>[2x]MSKNKVVIIGAGFAGLVAARELQTAGIEYEILEAKDRIGGRAWTEERMGRPLELGATWVHWFQAHTWTEIMRYGQRTEITASPSGNDAHWVTDGKVV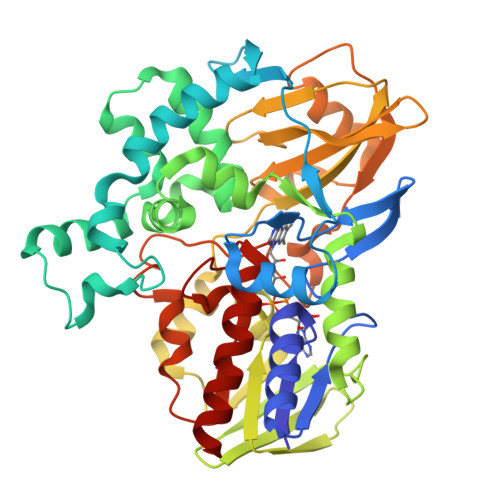KGTEDDLDEKLTAAMGVTYEGSEEYFPNPHDPLWVLSDDFDGPAEVRERFLSDDQTNAIDLVKEAGFDQETIDLVDAFWCAGYIGDPYTGSALMAKQWGALSDNRYRVMEDITLKWKLNNGMRSLYDGIAGDLNTDIRLNTPVAKVEHHDNGATVTTESGEVIEASAVICTVPVGALSNIEFSPALPDAVQSVIDDKWNSQGAKIWIKIKGHHRFLGYAPKPAKMSVVRSEYFMDDDTTILVGFGYDNTNIDLNSIEDAQAVINQWRDDLEVVDTTGHNWVADKWAGQAWGTLRKGQFTQGWSLFDDTDSQLFFAGSDYAYGWRGVSVDGALEKGMTTARQVINSMRETKEQ> GAMVPKASGTSGPAKQEKQSIITPADLLENMSPGWNLGNTLDAVPTEGSWNNPPVREHTFDDIRDAGFKSVRIPVTWDSHIGSAPEYPIDTDWMNRVEEVTDWALEREFYVVLNIHHDSWLWISRMGNSQQETLDKLGKVWKQIAERFKNKSERLLFEIVNEPTGMSAYQMNLLNREMLNIIRSTGGKNGQRLVIVGGLEDNKDELLHSFEPPDDDRIVLTYHYYSPWDYVSNWWGRTTWGSAAEISEMEEDIKPVYEKFVREGYPVIIGEYGTLGANEKHSKWLYHDTFVRLAHKYQMVPMWWDNGNDQFDRAERQWRDPVVKEIVIQAGRGVPNAIIKPADLFIKKGQSISDQTVDIQLNGNVLTGIYQKSEPLKEGSDYTVDNAGKTVSIKASCLAKLLNGAGQPGVKAQLTFTFHKGASQVMDIILYDDPKLEKSEFTISQSAISGDLKIPASLNGTKLATVKGVVDSTGRPVLEEVWSWTPYLNYDEDFYEKDGDLYLKERVLKYLKSDSTFTFELWPKGVEAVVKVKITP

Here, we report the crystal structure of a full-length GH5_4 enzyme from Bacillus licheniformis (BlCel5B) that exhibits two AMs (Ig-like module and CBM46) appended to the CD. The BlCel5B structure comprises three distinct domains: an N-terminal CD (residues 18 to 330), an Ig-like module (residues 335 to 428) and a family 46 CBM (residues 432 to 533). Full-length BlCel5B is active on both cellulosic and hemicellulosic substrates and auxiliary modules are crucial for its activity. We find that the large-scale conformational adjustments of the distal CBM46 mediated by the Ig-like hinge domain are crucial in active-site assembly for optimal substrate binding and hydrolysis.

BlCel5B crystals in the substrate-free form and complexed with cellopentaose (C5) were obtained and diffracted to 1.7 Å and 1.75 Å resolutions, respectively. The substrate-free and complexed structures exhibited no substantial conformational differences (with the exception of the substrate). Because of minor variations in the loops located distal to the substrate-binding site, a root mean squared deviation (rmsd) of 0.33 Å between the complexed and substrate-free structures was observed. A single protein chain occupies the asymmetric unit, and most of the residues were built, with the exception of the first 17 residues and those in the loop between L398 and P405 due to weak electron density. Similarly to other members of the GH5 family, the CD of BlCel5B has a typical TIM barrel fold with eight inner β-strands and eight outer α helices that are interconnected by loops and three short α helices. Very short linkers, D429-D430-P431 and V331-P332-N333-A334, connect the CBM46 to the Ig-like module and the Ig-like module to the CD, respectively. Both Ig-like module and CBM46 have a β-sandwich fold composed of two β-sheets of four and three antiparallel β-strands interconnected by loops and a short α helix between strands β3 and β4. In contrast, the CBM46 has three tryptophan residues, two of which face the CD substrate binding site, indicating that it may be actively engaged in the carbohydrate binding. The CD binding site of BlCel5B is open and relatively flat and is thus barely able to properly hold the substrate in position for catalysis without assistance from the CBM46. We found that the SAXS envelope can be well represented by considering the superimposition of three different representative molecular conformations of BlCel5B: a closed or CBM46/CD-occluded conformation extracted from the simulations with a relative weight of 26%, a semi-open conformation represented by the crystal structure corresponding to 40%, and an extended conformation based on simulations that is responsible for 34% of the SAXS envelope.> MSTPHHGRHELGQNFLSDRRVIADIVEIVSRTNGPIIEIGAGDGALTIPLQRLARPLTAVEVDARRARRLAQRTARSAPGPASRPTEVVAADFLRYPLPRSPHVVVGNLPFHLTTAILRRLLHGPGWTTAVLLMQWEVARRRAAVGGATMMTAQWWPWFEFGLARKVSAASFTPRPAVDAGLLTITRRSRPLVDVADRARYQALVHRVFTGRGHGMAQILQRLPTPVPRTWLRANGIAPNSLPRQLSAAQWAALFEQTRLT

Erythromycin resistance methyltransferases (Erms) confer resistance to macrolide, lincosamide, and streptogramin antibiotics in Gram-positive bacteria and mycobacteria. Using SAM as a cofactor, Erms transfer a methyl group to adenosine at position 2058 (A2058) in the ∼3000 nucleotide-long 23S ribosomal RNA. This subtle posttranscriptional modification blocks the antibiotic-binding site in the ribosomal peptide exit tunnel. Erm38 features at its N-terminal catalytic domain the classic Rossmann fold, an α/β sandwich that contains the SAM cofactor-binding site and a helical C-terminal domain.

Here, we present crystal structures of Erm38 from Mycobacterium smegmatis in apoprotein and cofactor-bound forms. Erm38 comprises 386 amino acids (NCBI WP_063844518; Uniport Q79N53), with analysis using the Database of Disordered Protein Predictions predicting that the N-terminal 12 residues and C-terminal 124 residues are disordered regions. We therefore expressed a truncated version of Erm38 spanning residues 13 to 261. This truncated Erm38, referred to as Erm38 throughout, has a molecular mass of 30 kDa and a size similar to most Erms from Gram-positive bacteria. The highly purified Erm38 formed square plate crystals that diffracted to a maximum resolution of 1.9 Å and tolerated up to 20% dimethylsulfoxide, which makes them suitable for ligand-soaking experiments. The electrostatic potential of Erm38 includes a highly positively charged region that comprises residues R119, R140, R141, R142, and K166 located at the protein surface. As these solvent-exposed basic residues are likely to be involved in binding the RNA substrate, we produced an alanine mutant for each site and compared the enzymatic activities of the mutant and WT enzymes. The E61K, R119A, R140A, and R141A mutations resulted in >90% reduction in methylation activity, whereas the R142A mutation resulted in 75% loss of enzymatic activity. One reason for the paucity of information about Erm-RNA structures is the adventitious precipitation of the Erm–RNA complex when the 32-mer RNA substrate is mixed with the apoprotein.> GSRISAEGSQACAKGCELCSEVNGCLKCSPKLFILLERNDIRQVGVCLPSCPPGY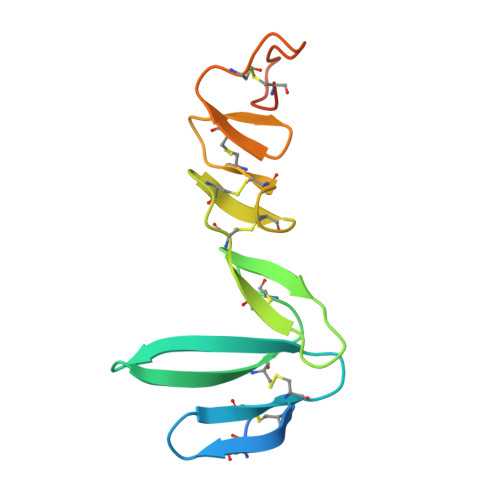FDARNPDMNKCIKCKIEHCEACFSHNFCTKCKEGLYLHKGRCYPACPEGSSAANGTMECSSPAAAHHHHHH> MRIIKPFAILTPQTIIQDKAVAFDKKIEAIDTVENLIKKYPNAAVEHDENSLLLPGFANPHLHLEFSANKATLQYGDFIPWLYSVIRHREDLLPLCDGACLEQTLSSIIQTGTTAIGAISSYGEDLQACIDSALKVVYFNEVIGSNAATADVMYASFLERFHQSKKHENERFKAAVAIHSPYSVHYILAKRA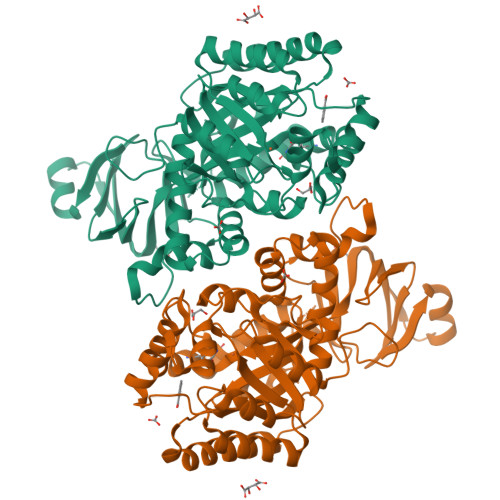LDIAKKYGSLVSVHFMESRAEREWLDKGSGEFAKFFKEFLNQTRPVNDTKSFLELFKELHTLFVHMVWANEEEIQTIASYNAHIIHCPISNRLLGNGVLDLEKIKSIPYAIATDGLSSNYSLNMYEELKAALFVHPNKEATTFAKELIIRATKAGYDALGFEGGEIAVGKDADMQLIDLPEGLTNVEDLYLHVILHTTKPKKVYIQGEEHVREAENLYFQSHHHHHHWSHPQFEK>[4x]GSGFEELPLCSCRMEAPKIDRISERAGHKCMATESVD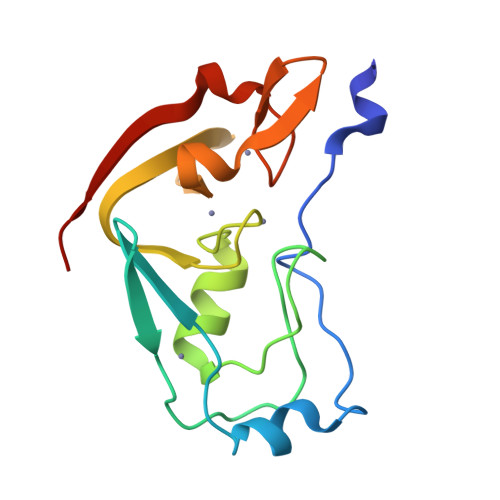GELSGCNAAILKRETMRPSSRVALMVLCETHRARMVKHHCCPGCGYFCTAGTFLECHPDFRVAHRFHKACVSQLNGMVFCPHCGEDASEAQEVTIPRGD>[2x]MSQTHKHAIPANIADRCLINPEQYETKYKQSINDPDTFWGEQGKILDWITPYQKVKNTSFAPGNVSIKWYEDGTLNLAANCLDRHLQENGDRTAIIWEGDDTSQSKHISYRELHRDVCRFANTLLDLGIKKGDVVAIYMPMVPEAAVAMLACARIGAVHSVIFGGFSPEAVAGRIIDSSSRLVITADEGVRAGRSIPLKKNVDDALKNPNVTSVEHVIVLKRTGS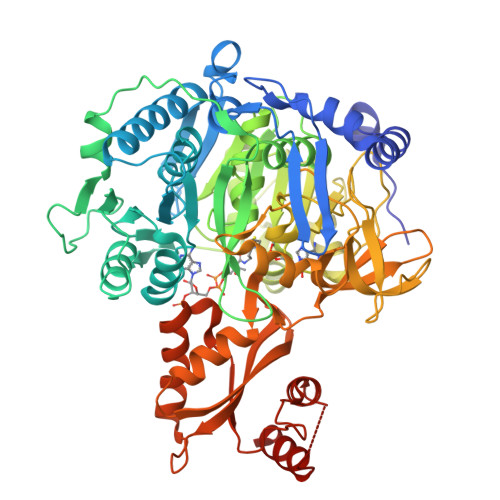DIDWQEGRDLWWRDLIEKASPEHQPEAMNAEDPLFILYTSGSTGKPKGVLHTTGGYLVYAATTFKYVFDYHPGDIYWCTADVGWVTGHSYLLYGPLACGATTLMFEGVPNWPTPARMCQVVDKHQVNILYTAPTAIRALMAEGDKAIEGTDRSSLRILGSVGEPINPEAWEWYWKKIGKEKCPVVDTWWQTETGGFMITPLPGAIELKAGSATRPFFGVQPALVDNEGHPQEGATEGNLVITDSWPGQARTLFGDHERFEQTYFSTFKNMYFSGDGARRDEDGYYWITGRVDDVLNVSGHRLGTAEIESALVAHPKIAEAAVVGIPHAIKGQAIYAYVTLNHGEEPSPELYAEVRNWVRKEIGPLATPDVLHWTDSLPKTRSGAIMRRILRKIAAGDTSNLGDTSTLADPGVVEKLLEEKQAIAMPS> WKYWR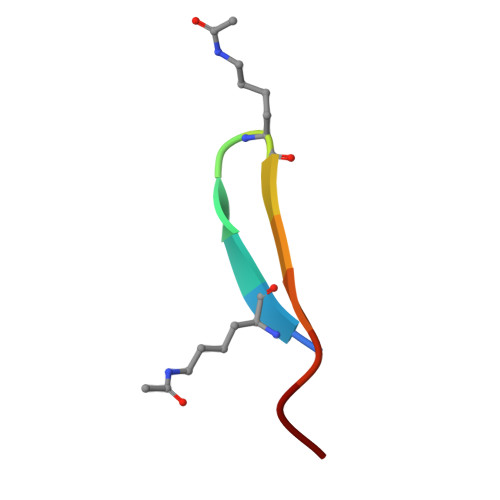KYVLKIC>[4x]MHHHHHHENLYFQSSSQFHGLAIGNGNSNYLQVLGLANITDTAYLTDWQDSGGNWHAGFALPVPSDYPKGHFFQLTTGVGNSNYLQVLGAGEDGNPYLVSWQDGSGKWHGGMPLPKPSGYSGGPLVTGIGNSNYLQVIGARVESSPYLVAWQDNGGNWHAGMPLPNPSGYAGGFQQLATGNGNDHFLQVVGVGNDGN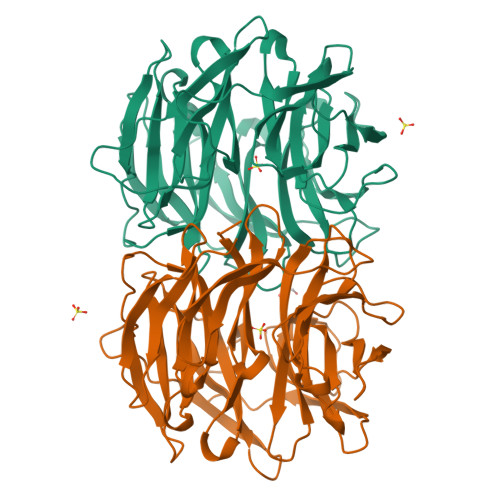AYLVTWQNAQGQWSPGFALPKPSGYSGTFTQLATGVGNGNFLQVLGIGTDGNAYLVAWQDNGGNWHPGFALPKPSGYNGTFAKLVTGIGNSNYLQVFGIGSNGVAYLVSWQDSGGNWHGGLTLPQPSGYNGSFSQLAAGNGNSHYLQVVGTDAQGNVYLVSWQDSEGKWHAGFELPRAS>MADYKDDDDKSGRMLNNLTDCEDGDGGANPGDGNPKESSPFINSTDTEKGKEYDGKNMALFEEEMDTSPMVSSLLSGLANYTNLPQGSREHEEAENNEGGKKKPVQAPRMGTFMGVYLPCLQNIFGVILFLRLTWVVGIAGIMESFCMVFICCSCTMLTAISMSAIATNGVVPAGGSYYMISRSLGPEFGGAVGLCFYLGTTFAGAMYILGTIEILLAYLFPAMAIFKAEDASGEAAAMLNNMRVYGTCVLTCMATVVFVGVKYVNKFALVFLGCVILSILAIYAGVIKSAFDPPNFPICLLGNRTLSRHGFDVCAKLAWEGNETVTTRLWGLFCSSRFLNATCDEYFTRNNVTEIQGIPGAASGLIKENLWSSYLTKGVIVERSGMTSVGLADGTPIDMDHPYVFSDMTSYFTLLVGIYFPSVTGIMAGSNRSGDLRDAQKSIPTGTILAIATTSAVYISSVVLFGACIEGVVLRDKFGEAVNGNLVVGTLAWPSPWVIVIGSFFSTCGAGLQSLTGAPRLLQAISRDGIVPFLQVFGHGKANGEPTWALLLTACICEIGILIASLDEVAPILSMFFLMCYMFVNLACAVQTLLRTPNWRPRFRYYHWTLSFLGMSLCLALMFICSWYYALVAMLIAGLIYKYIEYRGAEKEWGDGIRGLSLSAARYALLRLEEGPPHTKNWRPQLLVLVRVDQDQNVVHPQLLSLTSQLKAGKGLTIVGSVLEGTFLENHPQAQRAEESIRRLMEAEKVKGFCQVVISSNLRDGVSHLIQSGGLGGLQHNTVLVGWPRNWRQKEDHQTWRNFIELVRETTAGHLALLVTKNVSMFPGNPERFSEGSIDVWWIVHDGGMLMLLPFLLRHHKVWRKCKMRIFTVAQMDDNSIQMKKDLTTFLYHLRITAEVEVVEMHESDISAYTYEKTLVMEQRSQILKQMHLTKNEREREIQSITDESRGSIRRKNPANTRLRLNVPEETAGDSEEKPEEEVQLIHDQSAPSCPSSSPSPGEEPEGEGETDPEKVHLTWTKDKSVAEKNKGPSPVSSEGIKDFFSMKPEWENLNQSNVRRMHTAVRLNEVIVKKSRDAKLVLLNMPGPPRNRNGDENYMEFLEVLTEHLDRVMLVRGGGREVITIYS[2x]

The electroneutral K+-Cl− cotransporters (KCCs) play fundamental roles in trans-epithelial transport, cell volume regulation, and neuronal excitability. The neuronal-specific KCC2 (SLC12A5) and glial-expressed KCC3 (SLC12A6) are essential for normal development and function of the nervous system. Here, we present single particle cryo-electron microscopy (cryo-EM) structures of the full-length human KCC2 and KCC3 at overall resolution of 3.2 and 3.3 Å, respectively. The structures of KCC2 and KCC3 are very similar to each other.

In the cryo-EM map of KCC2, the densities for K+ and one of Cl− ions are absent. The corresponding N-terminal loop of KCC2 (residues A65-N83) is also bound in the same location with the same mode as KCC3, consist with the sequence conservation in this region. The N-terminal loop of KCC2/3 binds to the intracellular vestibule of the transporter, arresting the transporters in an inhibited state. In conclusion, we solved the cryo-EM structures of KCC2 and KCC3, which display a distinct configuration compared to NKCC1.>[4x]MHHHHHHMISGSVRFLVNLESLNGVESIGNLTKHRTAPVVLKTSTGYLVRYVPVISGEALAHAYQASLVDIAKKEGLPVGSLSSQYEFIKFSTDEALKIEGIKEPKDYNDARRFEVEVMLKDVIADVGGFMYAGGAPVRRTSRIKLGYMIPALRGDEIPAQLEAQFHVRFSNKPVSGSQAIFNVEVSSA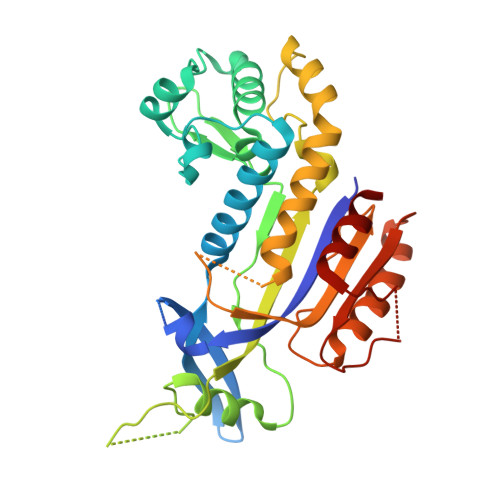LYTFSFELDEDLIAVPSTFGEKVKGEEELERQKAKRVKSAIKALYSLLSGNFGGKRSRFLPSMKLMSLVVTKTDFPFMPEPAHDDDYIKTTIMRLGKAKGVLNGNLAKAYVINNEGIEVGEGVTVLSTVEDLVVKLEEE> SMTSSANEDMPVERILEAELAVEPKTETYVEANMGLNPSSPNDPVTNICQAADKQLFTLVEWAKRIPHFS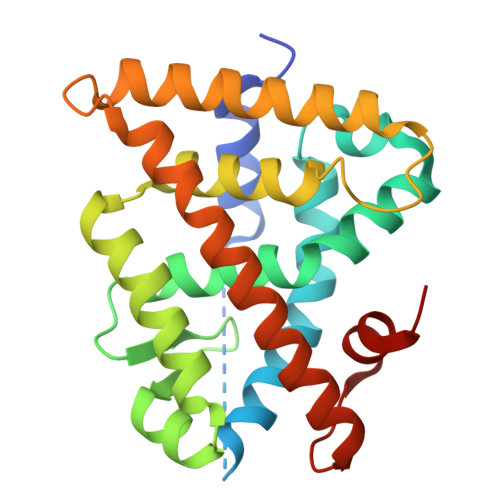ELPLDDQVILLRAGWNELLIASFSHRSIAVKDGILLATGLHVHRNSAHSAGVGAIFDRVLTELVSKMRDMQMDKTELGCLRAIVLFNPDSKGLSNPAEVEALREKVYASLEAYCKHKYPEQPGRFAKLLLRLPALRSIGLKCLEHLFFFKLIGDTPIDTFLMEMLEAPHQMT>[3x]TTIVSVRRNGQVVVGGDGQVSLGNTVMKGNARKVRRLYNGKVLAGFAGGTADAFTLFELFERKLE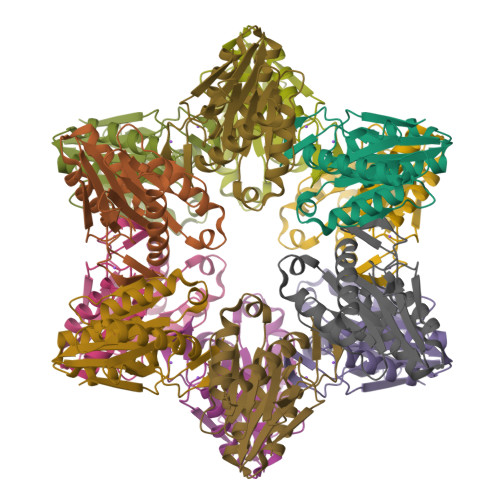MHQGHLLKSAVELAKDWRTDRALRKLEAMLIVADEKESLIITGIGDVVQPEEDQILAIGSGGNYALSAARALVENTELSAHEIVEKSLRIAGDICVFTNTNFTIEELPN2-{[2-chloro-5-(trifluoromethyl)phenyl]amino}-5-methoxybenzoic 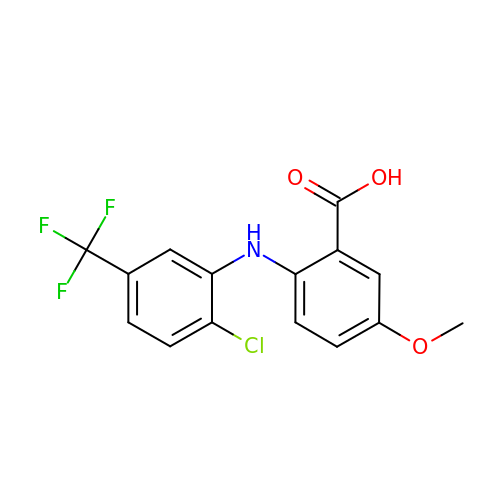acid | C15 H11 Cl F3 N O3 | FYBDCWMCUHIQSM-UHFFFAOYSA-N> MPTTFDDILEHIGEFGRFQKQTFFLLCLLSAAFAPIYVGIVFLGFTPDHRCRSPGVAELSQRCGWSLEEELNYTVPGVGSSGEASPSQCRRYEVDWNQTGLSCTDPLASLAANRSHLPLGPCQDGWVYDTPGSSIVTEFNLVCADSWMLDLVQAAVNVGFFVGSMSIGYIADRFGRKLCLLVTILINAISGVLMAVAPNYTWMLIFRLIQGLVSKGGWLIGYTLPTEFVGLEYRRTVGILYQMAFSVGLLVLAGVAYAIPHWRWLQLAVTLPNFFFLLYYWCIPESPRWLISQNKNAKAMKIIKHIAKKN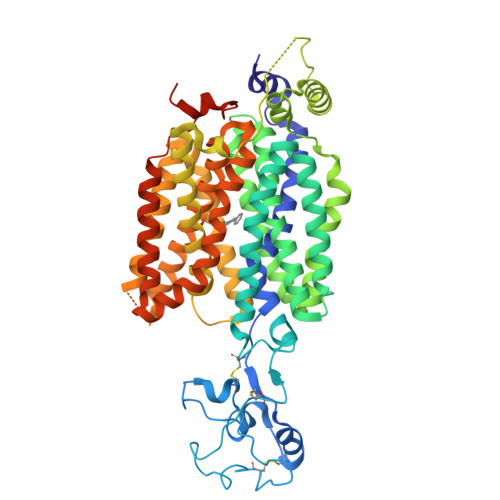GKKLPKSLQEERKETEVGEKLNPSFLDLVRTPQIRKHTLILMYNWFTSSVLYQGLIMHMGIAGGNIYLDFFYSALVEFPAAFIIILTIDRIGRRYPWAAANMVAGAACLITAFIPDGLFWLKTTVACLGRMGITMAFEMVCFVNTELYPTFIRNLGVLVCSSLCDIGGIITPFLVYRLASIWLELPLVVFAVLGLIAGGLVLLLPETKGKPLPETIEDAENPHRPRKNKEKMIYLQVLLSDIPDN>MAKNVGILAMDIYFPPTCVQQEALEAHDGASKGKYTIGLGQDCLAFCTELEDVISMSFNAVTSLLEKYKIDPKQIGRLEVGSETVIDKSKSIKTFLMQLFEKCGNTDVEGVDSTNACY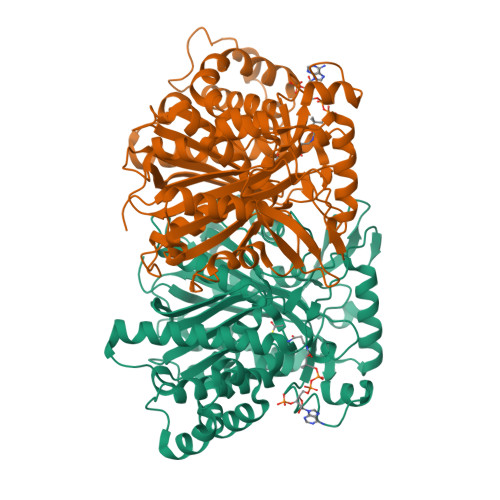GGTAALLNCVNWVESNSWDGRYGLVICTDSAVYAEGPARPTGGAAAIAMLIGPDAPIVFESKLRGSHMAHVYDFYKPNLASEYPVVDGKLSQTCYLMALDSCYKHLCNKFEKLEGKEFSINDADYFVFHSPYNKLVQKSFARLLYNDFLRNASSIDEAAKEKFTPYSSLSLDESYQSRDLEKVSQQLAKTYYDAKVQPTTLVPKQVGNMYTASLYAAFASLVHNKHSDLAGKRVVMFSYGAGSTATMFSLRLCENQSPFSLSNIASVMDVGGKLKARHEYAPEKFVETMKLMEHRYGAKEFVTSKEGILDLLAPGTYYLKEVDSLYRRFYGKKGDDGSITNGH[4x]(2Z)-1-[(6-chloropyridin-3-yl)methyl]imidazolidin-2-imine 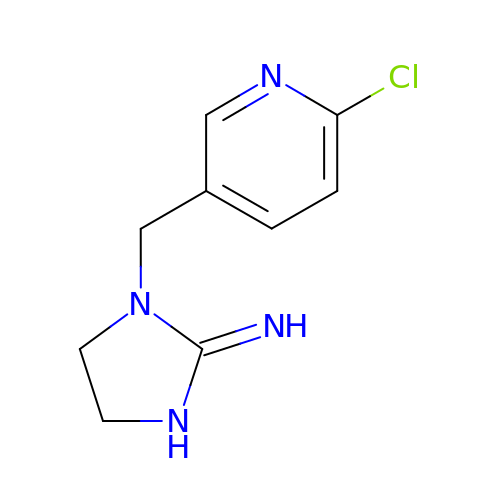| C9 H11 Cl N4 | UEQZFAGVRGWPDK-UHFFFAOYSA-N> AGGHGDVGMHVKEKEKNKDENKRKDEERNKTQEEHLKEIMKHIVKIEVKGEEAVKKEAAEKLLEKVPSDVLEMYKAIGGKIYIVDGDITKHISLEALSEDKKKIKDIYGKDALLHEHYVYAKEGYEPVLVIQSSEDYVENTEKALNVYYEIGKILSRDILSKINQPYQKFLDVLNTIKNASDSDGQDLLFTNQLKEHPTDFSVEFLEQNSNEVQEVFAKAFAYYIEPQHRDVLQLYAPEAFNYMDKFNEQEINLSLEELKDQRMLSRYEKWEKIKQHYQHWSDSLSEEGRGLLKKLQIPIEPKKDDIIHSLSQEEKELLKRIQIDSSDFLSTEEKEFLKKLQIDIRDSLSEEEKELLNRIQVDSSNPLSEKEKEFLKKLKLDIQPYDINQRLQDTGGLIDSPSINLDVRKQYKRDIQNIDALLHQSIGSTLYNKIYLYENMNINNLTATLGADLVDSTDNTKINRGIFNEFKKNFKYSISSNYMIVDINERPALDNERLKWRIQLSPDTRAGYLENGKLILQRNIGLEIKDVQIIKQSEKEYIRIDAKVVPKSKIDTKIQEAQLNINQEWNKALGLPKYTKLITFNVHNRYASNIVESAYLILNEWKNNIQSDLIKKVTNYLV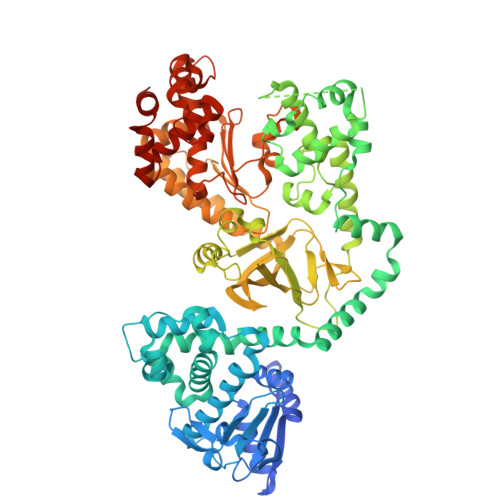DGNGRFVFTDITLPNIAEQYTHQDEIYEQVHSKGLYVPESRSILLHGPSKGVELRNDSEGFIHEFGHAVDDYAGYLLDKNQSDLVTNSKKFIDIFKEEGSNLTSYGRTNEAEFFAEAFRLMHSTDHAERLKVQKNAPKTFQFINDQIKFIINS>GHMAKTYDYLFKLLLIGDSGVGKTCVLFRFSEDAFNSTFISTIGIDFKIRTIELDGKRIKLQIWDTAGQERFRTITTAYYRGAMGIMLVYDITNEKSFDNIRNWIRNIEEHASADVEKMILGNKCDVNDKRQVSKERGEKLALDYGIKFMETSAKANINVENAFFTLARDIKAKMDKKLEGNSPQG[2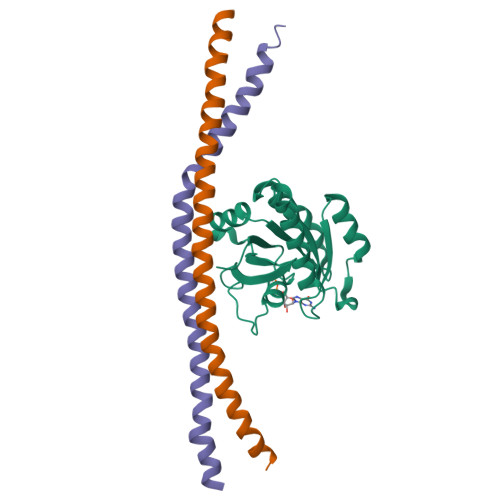x];>GPGYERLKEELAKAQRELKLKDEECERLSKVRDQLGQELEELTASLFEEAHKMVREANIKQATAEKQLKEAQGKIDVL[4x]methyl (6-cyano-3-{2-[2-(2,4-dioxo-3,4-dihydropyrimidin-1(2H)-yl)ethoxy]phenoxy}-4-methylnaphthalen-1-yl)acetate 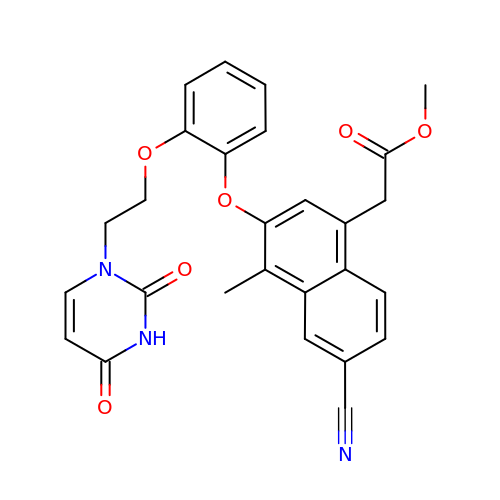| C27 H23 N3 O6 | NMVRVCAJVLRWGN-UHFFFAOYSA-N>GAMADIGSDSEDEFPEITEEMEKEIKNVFRNGNQDEVLSEAFRLTITRKDIQTLNHLNWLNDEIINFYMNMLMERSKEKGLPSVHAFNTFFFTKLKTAGYQAVKRWTKKVDVFSVDILLVPIHLGVHWCLAVVDFRKKNITYYDSMGGINNEACRILLQYLKQESIDKKRKEFDTNGWQLFSKKSQEIPQQMNGSDCGM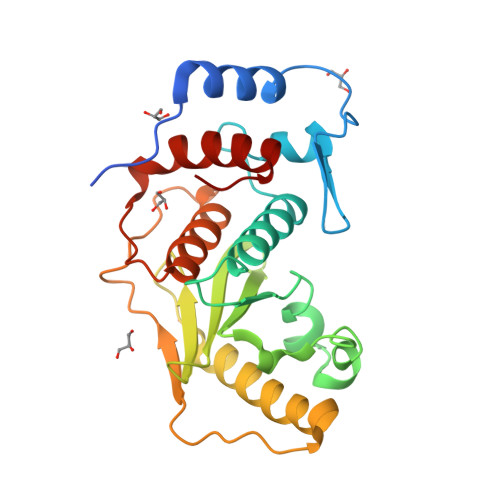FACKYADCITKDRPINFTQQHMPYFRKRMVWEILHRKLL[2x]Most eukaryotic messenger RNAs (mRNAs) are processed at their 3′ end by the cleavage and polyadenylation specificity factor (CPF/CPSF). CPF mediates the endonucleolytic cleavage of the pre-mRNA and addition of a polyadenosine (poly(A)) tail, which together define the 3′ end of the mature transcript. In the yeast Saccharomyces cerevisiae, CPF is assembled into a 14-subunit (∼850 kDa) complex, which is organized into three enzymatically distinct and interconnected modules: the polymerase, nuclease, and phosphatase modules (Casañal et al., 2017). The nuclease module contains the endonuclease Ysh1, the pseudo-nuclease Cft2, and the multidomain protein Mpe1 (orthologs of human CPSF73, CPSF100, and RBBP6, respectively).

Compared with the previous structure of the yeast polymerase module (Casañal et al., 2017), the sample we used here additionally contained Pap1, Mpe1, and the precleaved CYC1 RNA. We obtained a map of the complex at an overall resolution of 2.7 Å. In this map, we identified an additional density, which is not present in the previous maps of the yeast polymerase module or mPSF (Casañal et al., 2017; Zhang et al., 2020), that extends from the top of Pfs2 toward Yth1 and Cft1 (orange). Given the resolution of the map, we could de novo build an atomic model into a part of the additional density, including a region of Mpe1 downstream of the zinc knuckle (residues 207–222 and 240–268). We will refer to the region of Mpe1 that is ordered in our maps as the pre-mRNA-sensing region (PSR). Mpe1 residues 207–252 form a small, compact fold that packs against the Pfs2 beta-propeller. Mpe1 then continues as a helix (residues 253–268) that makes additional contacts with the side of the Pfs2 beta-propeller. Two aromatic residues from this helix (W257 and Y260) insert into a hydrophobic pocket of Pfs2 that is lined by W149, I161, and F206. The density near the zinc finger 2 of Yth1 corresponds to the nucleotides A1 and A2 of the PAS of CYC1 (A1A2G3A4A5), as well as one additional upstream nucleotide (U−1). Surprisingly, in addition to the interactions between RNA and Yth1, A2 is contacted directly by P215 of Mpe1 through a CH-π interaction (Levitt and Perutz, 1988).

> MNVYDDVLDATVVSHSLATHFTTSDYEELLVVRTNILSVYRPTRDGKLYLTDEFKFHGLITDIGLIPQKDSPLSCLLLCTGVAKISILKFNTLTNSIDTLSLHYYEGKFKGKSLVELAKISTLRMDPGSSCALLFNNDIIAFLPFHVNKNDDDEEEEDEDENIDDSELIHSMNQKSQGTNTFNKRKRTKLGDKFTAPSVVLVASELYEGAKNIIDIQFLKNFTKPTIALLYQPKLVWAGNTTISKLPTQYVILTLNIQPAESATKIESTTIAFVKELPWDLHTIVPVSNGAIIVGTNELAFLDNTGVLQSTVLLNSFADKELQKTKIINNSSLEIMFREKNTTSIWIPSSKSKNGGSNNDETLLLMDLKSNIYYIQMEAEGRLLIKFDIFKLPIVNDLLKENSNPKCITRLNATNSNKNMDLFIGFGSGNALVLRLNNLKSTIETREAHNPSSGTNSLMDINDDDDEEMDDLYADEAPENGLTTNDSKGTVETVQPFDIELLSSLRNVGPITSLTVGKVSSIDDVVKGLPNPNKNEYSLVATSGNGSGSHLTVIQTSVQPEIELALKFISITQIWNLKIKGRDRYLITTDSTKSRSDIYESDNNFKLHKGGRLRRDATTVYISMFGEEKRIIQVTTNHLYLYDTHFRRLTTIKFDYEVIHVSVMDPYILVTVSRGDIKIFELEEKNKRKLLKVDLPEILNEMVITSGLILKSNMCNEFLIGLSKSQEEQLLFTFVTADNQIIFFTKDHNDRIFQLNGVDQLNESLYISTYQLGDEIVPDPSIKQVMINKLGHDNKEEYLTILTFGGEIYQYRKLPQRRSRFYRNVTRNDLAITGAPDNAYAKGVSSIERIMHYFPDYNGYSVIFVTGSVPYILIKEDDSTPKIFKFGNIPLVSVTPWSERSVMCVDDIKNARVYTLTTDNMYYGNKLPLKQIKISNVLDDYKTLQKLVYHERAQLFLVSYCKRVPYEALGEDGEKVIGYDENVPHAEGFQSGILLINPKSWKVIDKIDFPKNSVVNEMRSSMIQINSKTKRKREYIIAGVANATTEDTPPTGAFHIYDVIEVVPEPGKPDTNYKLKEIFQEEVSGTVSTVCEVSGRFMISQSQKVLVRDIQEDNSVIPVAFLDIPVFVTDSKSFGNLLIIGDAMQGFQFIGFDAEPYRMISLGRSMSKFQTMSLEFLVNGGDMYFAATDADRNVHVLKYAPDEPNSLSGQRLVHCSSFTLHSTNSCMMLLPRNEEFGSPQVPSFQNVGGQVDGSVFKIVPLSEEKYRRLYVIQQQIIDRELQLGGLNPRMERLANDFYQMGHSMRPMLDFNVIRRFCGLAIDRRKSIAQKAGRHAHFEAWRDIINIEFSMRSLCQGK;> MSLIHPDTAKYPFKFEPFLRQEYSFSLDPDRPICEFYNSREGPKSCPRGPLCPKKHVLPIFQNKIVCRHWLRGLCKKNDQCEYLHEYNLRKMPECVFFSKNGYCTQSPDCQYLHIDPASKIPKCENYEMGFCPLGSSCPRRHIKKVFCQRYMTGFCPLGKDECDMEHPQFIIPDEGSKLRIKRDDEINTRKMDEEKERRLNAIINGEV;> MDGHNQNQYQNQNQIQQSQQPPLKKYVTQRRSVDVSSPYINLYYNRRHGLPNLVVEPETSYTIDIMPPNAYRGRDRVINLPSKFTHLSSNKVKHVIPAIQWTPEGRRLVVATYSGEFSLWNASSFTFETLMQAHDSAVTTMKYSHDSDWMISGDADGMIKIWQPNFSMVKEIDAAHTESIRDMAFSSNDSKFVTCSDDNILKIWNFSNGKQERVLSGHHWDVKSCDWHPEMGLIASASKDNLVKLWDPRSGNCISSILKFKHTVLKTRFQPTKGNLLMAISKDKSCRVFDIRYSMKELMCVRDETDYMTLEWHPINESMFTLACYDGSLKHFDLLQNLNEPILTIPYAHDKCITSLSYNPVGHIFATAAKDRTIRFWTRARPIDPNAYDDPTYNNKKINGWFFGINNDINAVREKSEFGAAPPPPATLEPHALPNMNGFINKKPRQEIPGIDSNIKSSTLPGLSI;> MSSTIFYRFKSQRNTSRILFDGTGLTVFDLKREIIQENKLGDGTDFQLKIYNPDTEEEYDDDAFVIPRSTSVIVKRSPAIKSFSVHSRLKGNVGAAALGNATRYVTGRPRVLQKRQHTATTTANVSGTTEEERIASMFATQENQWEQTQEEMSAATPVFFKSQTNKNSAQENEGPPPPGYMCYRCGGRDHWIKNCPTNSDPNFEGKRIRRTTGIPKKFLKSIEIDPETMTPEEMAQRKIMITDEGKFVVQVEDKQSWEDYQRKRENRQIDGDETIWRKGHFKDLPDDLKCPLTGGLLRQPVKTSKCCNIDFSKEALENALVESDFVCPNCETRDILLDSLVPDQDKEKEVETFLKKQEELHGSSKDGNQPETKKMKLMDPTGTAGLNNNTSLPTSVNNGGTPVPPVPLPFGIPPFPMFPMPFMPPTATITNPHQADASPKK>[3x]MEKQNIAVILARQNSKGLPLKNLRKMNGISLLGHTINAAISSKCFDRIIVSTDGGLIAEEAKNFGVEVVLRPAELASDTASSISGVIHALETIGSNSGTVTLLQPTSPLRTGAH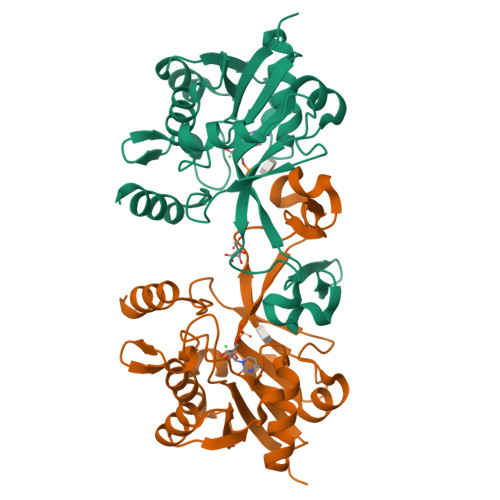IREAFSLFDEKIKGSVVSACPMEHHPLKTLLQINNGEYAPMRHLSDLEQPRQQLPQAFRPNGAIYINDTASLIANNCFFIAPTKLYIMSHQDSIDIDTELDLQQAENILNHKES>SNSKEITAQSQRHILNQSDHLRIDYELTRESMTKLRLVIFYSNISSDPITNFALL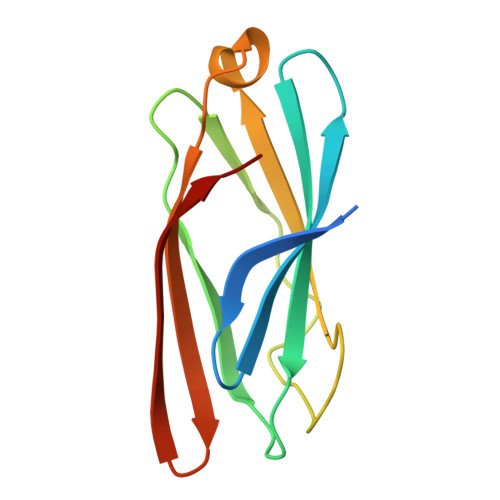VASPKGTTLSLQPQSGNMLQSNSRDGIKQIASVEGISVNLGKPIKLKWKANYCTKGDSKEESGTTSLPTI[4x]> MIIPALDLI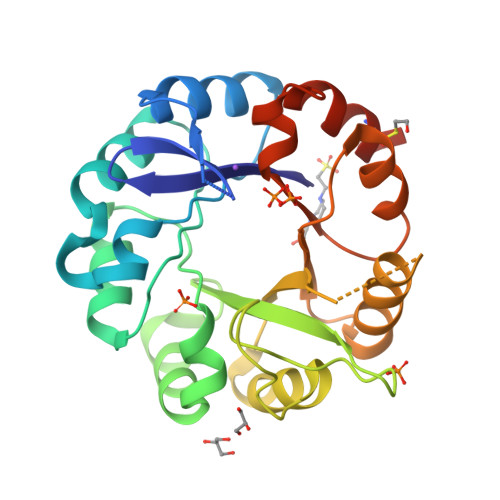DGTVVRLHQGDYARQRDYGNDPLPRLQDYAAQGAGVLHLVDLTGAKDPAKRQIPLIKTLVAGVNVPVQVGGGVRTEEDVAALLKAGVARVVIGSTAVKSPDVVKGWFERFGAQALVLALDVRIDEHGTKQVAVSGWQENSGVSLEQLVETYLPVGLKHVLCTDISRDGTLAGSNVSLYEEVCARYPQIAFQSSGGIGDIDDIAALRGTGVRGVIVGRALLEGKFTVKEAIQCWQNVKGHHHHHH5-hydroxy-6-methyl-4-oxo-4H-pyran-2-carboxylic 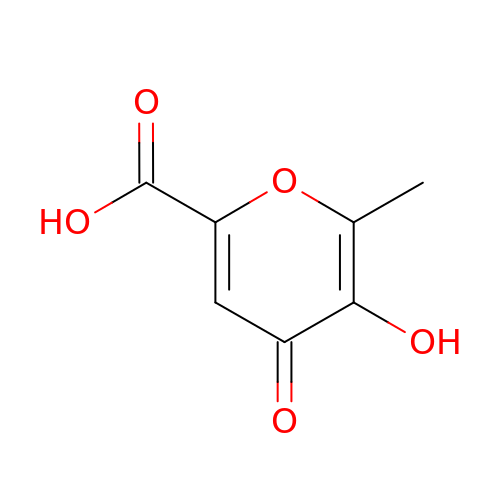acid | C7 H6 O5 | ANRPPKUCFMTTIH-UHFFFAOYSA-N>[2x]MRQATVYIDRQALQYNLNRVKQLAANSKIVSMVKANAYGHGVKDCLAALNASDAFGVACLQEGLEIRELGFEQPVTLIEGVFSEDEMPVAIEQKFECVIHHQQQFEWLIKHKQAYIAQGLKVWVKLNSGMNRLGFKDPEIIEVIKTLKSEGFTCVLAMHFANADVDHPLNEQQKQQFLHIKETCDPILASCCNSAAIFKWPELNFDYVRPGIMLYGASPFADKTVHDLDLKPVMTFTAEIIALNHIEAGEHVGYGSTFCAQQAMDIAIVSIGYGDGYPRAYVKQNFVAIDGKLCPVVGRVSMDMIAIDVTNTQVKLGTQVELWGNHRLVDDVAEANGTIGYELLCRLSSRPVRQGT

Alanine racemase (EC 5.1.1.1) is a pyridoxal 5′-phosphate (PLP)-dependent enzyme which catalyses racemization between l-alanine and d-alanine. d-Alanine is an essential building block of peptidoglycan, a critical component of the bacterial cell wall. Alanine racemase (Alr) is the sole source of d-alanine in many bacteria and its inhibition is lethal, making the enzyme an attractive antibiotic drug target. Kinetic studies of Alr have indicated that racemization occurs via a stepwise two-base mechanism, in which a highly conserved lysine and a tyrosine residue act as acid and base catalysts. Each Alr monomer has two distinct domains: an α/β-barrel at the N-terminus and a predominantly β-stranded domain at the C-terminus.

We have reported the crystal structure of A. baumannii alanine racemase from the highly antibiotic-resistant NCTC13302 strain to 1.9 Å resolution. The tertiary structure of A. baumannii alanine racemase (AlrAba) is a homodimer in which the two monomers interact in a head-to-tail manner. The individual AlrAba monomers are crystallographically distinct and form a dimer in the asymmetric unit. Overall, the AlrAba structure is lacking clear density for residues 247–263 and 355–356 of monomer B. Missing density for these regions has previously been observed in alanine racemases from other species, including M. tuberculosis, B. henselae, S. aureus and O. oeni. The essential PLP cofactor is covalently bound to Lys34 via an internal aldimine linkage and extends towards the centre of the α/β-barrel. The pyridine N1 of the PLP ring is stabilized by hydrogen bonding to Arg209, which is further stabilized by interactions with His159. Arg132 usually interacts with the phenolic O atom (O3′) of PLP, aiding in maintaining the position of the cofactor. However, Arg132 was not within hydrogen-bonding distance of PLP in the AlrAba structure. The lack of substrate-like molecules in the active site could also be a contributory factor to the unusual position of Arg132 owing to this residue playing an integral role in substrate binding. AlrAba has a hinge angle of 141.6°, identical to that of DadXPao (141.6°) and very similar to that of AlrEco (140.4°), to which it has the most similar active-site architecture.>MTEPSLSPAVQTFWKWLQEEGVITAKTPVKASVVTEGLGLVALKDISRNDVILQVPKRLWINPDAVAASEIGRVCSELKPWLSVILFLIRERSREDSVWKHYFGILPQETDSTIYWSEEELQELQGSQLLKTTVSVKEYVKNECLKLEQEIILPNKRLFPDPVTLDDFFWAFGILRS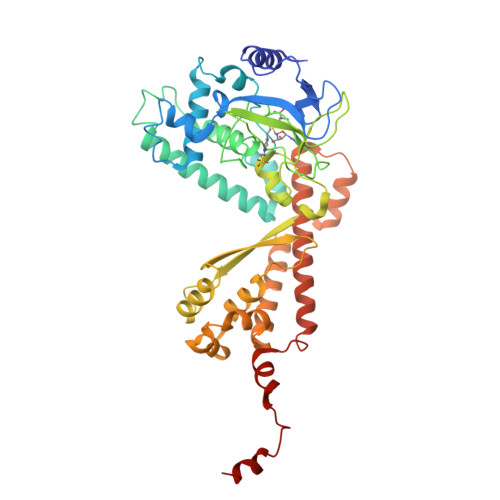RAFSRLRNENLVVVPMADLINHSAGVTTEDHAYEVKGAAGLFSWDYLFSLKSPLSVKAGEQVYIQYDLNKSNAELALDYGFIEPNENRHAYTLTLEISESDPFFDDKLDVAESNGFAQTAYFDIFYNRTLPPGLLPYLRLVALGGTDAFLLESLFRDTIWGHLELSVSRDNEELLCKAVREACKSALAGYHTTIEQDRELKEGNLDSRLAIAVGIREGEKMVLQQIDGIFEQKELELDQLEYYQERRLKDLGLCGENGDILENLYFQ[3x]~{N}-[3-(5-ethanoyl-2-ethoxy-phenyl)-5-(2-ethyl-5-methyl-3-oxidanylidene-1,2-oxazol-4-yl)phenyl]furan-2-carboxamide 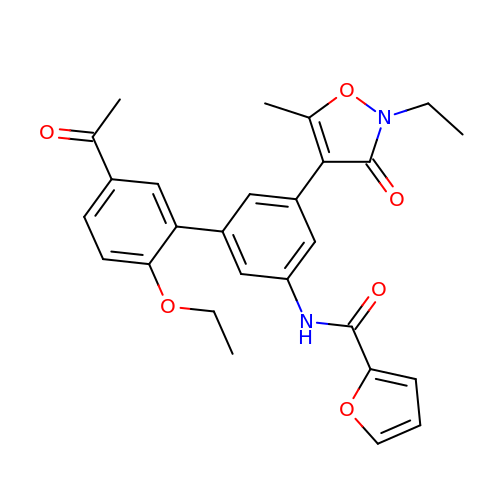| C27 H26 N2 O6 | HJDBFGUURXLNGK-UHFFFAOYSA-N> MLRSRVTGVVLAAGYSRRLGTPKQLLPLGDTTLLGATLAMARRCPFDQLIVTLGGAADEVLEKVELDGLDIVLVDDAGLGCSSSLKSALTWVDPTAEGIVLMLGDQPGITASAVASLIAGGRGATIAVCEYANGIGHPFWVSRGVFGDLAELHGDKGVW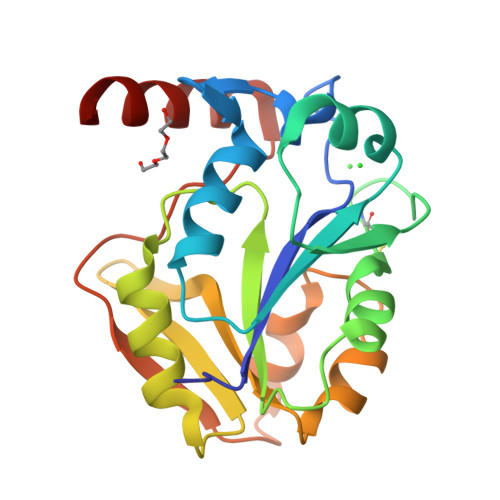RLIESGRHGVRRIRVDADVPLDVDTWDDYERLLASVVRLE>MKRIYIFLLCFAVLLPVGGKTAQAKEQAGEQYLLLEHVKDKSKLLDTAEQFHIHADVIEEIGFAKVTGEKQKLAPFTKKLAEKVGADVIEKPIANTAVNE[8x];>[8x]TESVISGSPAWGLDGILELKEYLWFAAKQTDSYRTYQIERGHPDVKVALIDSGLDLDHPDLKASVNTNGGWNYIDGKPVSGDPTGHGTQTAGMINIIAPDVTITPYQVLDEKGGDSYNIMKAMVDAVNDGHEVINISTGSYTSLDREGKVLMKAYQRAANYAAKHQVLVFSSAGNKGVNLDEMRKTE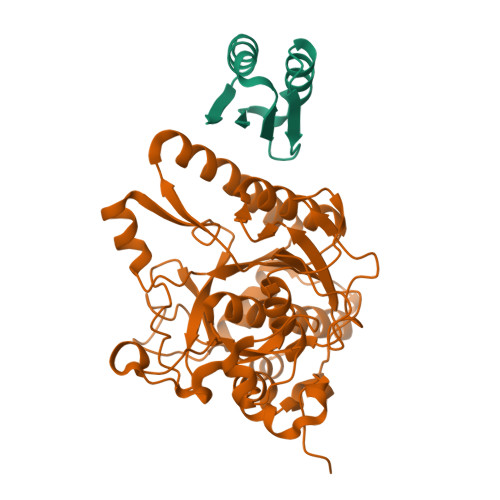NKVHLPSALKHVVSVGSNMKSNNISPYSNQGREIEFTAPGGYLGETYDQDGMVRVTDLVLTTYPKGKDNTALDQMLNIPKGYSLSYGTSLAAPQVAGTAALVISEYRERHHRKPSAKQVHHILRKSALDLGKPGKDVIYGYGEVRAYQALKMMNKE Meiosis arrest female 1 (MARF1) is a cytoplasmic RNA binding protein that is essential for meiotic progression of mouse oocytes, in part by limiting retrotransposon expression. Human MARF1 contains a NYN-like domain, two RRMs and eight LOTUS domains. Thus, MARF1 post-transcriptionally represses gene expression by serving as both an endoribonuclease and as a platform that recruits the DCP1:DCP2 decapping complex to targeted mRNAs.

To gain structural insights into the MARF1 NYN domain, we crystallized a human MARF1 protein construct encompassing amino acid residues 352–500 and determined its structure at a resolution of 1.7 Å by single-wavelength anomalous diffraction. Although the NYN domain crystallized as a dimer in the asymmetric unit of the crystal, both the wild-type NYN domain and the mutated protein used for crystallization (I391M/L457M) are monomeric in solution, as determined by size exclusion chromatography. The MARF1 NYN domain consists of a central six-stranded parallel beta-sheet flanked by pairs of alpha-helices on both sides, in contrast to the previously determined structure of the NYN domain of Bacillus subtilis YacP/Rae1, whose central beta-sheet contains only five strand. Despite lack of extensive sequence conservation, the MARF1 NYN domain exhibits substantial structural similarity to canonical PIN domains of ribonucleases MCPIP1 (39) and SMG6 (40), superimposing with root-mean-square deviations of 3.0 Å (over 96 Cα atoms) and 3.4 Å (94 Cα atoms), respectively. A prominent feature of the molecular surface of the MARF1 NYN domain is a highly conserved negatively charged patch formed by Asp358, Asp426, Asp427 and Asp452. Similar clusters of acidic amino acids define the active sites of PIN domain ribonucleases, including SMG6 and MCPIP1, in which they coordinate a divalent metal ion that in turn coordinates the substrate RNA and activates a water molecule for nucleophilic attack on the scissile phosphodiester group. Importantly, these amino acids are strictly conserved in MARF1 orthologs and map to equivalent residues in the SMG6 and MCPIP1 domain structures. Crucially these residues are not present in the SMG5 PIN domain, which has been shown to lack RNase activity. Together, these structural observations strongly suggest that the MARF1 NYN domain is a catalytically competent ribonuclease. In order to determine whether residues in the active site pocket are important for NYN enzymatic activity, we generated a NYN mutant in which Asp426 and 427 were mutated in tandem to alanines (NYNMUT). The nuclease activity of NYNMUT was strongly reduced as compared to NYNWT.

>GPLGSPIGVFWDIENCSVPSGRSATAVVQRIREKFFKGHREAEFMCVCDISKENKEVIQELNNCQVTVAHINATAKNAADDKLRQSLRRFANTHTAPATVVLVSTDVNFAMELSDLRHRHGFHIILVHKNQASEALLHHANELIRFEEFISDLPHHHHHH[2x]3-(3-bromobenzyl)-1-tert-butyl-1H-pyrazolo[3,4-d]pyrimidin-4-amine | C16 H18 Br N5 | 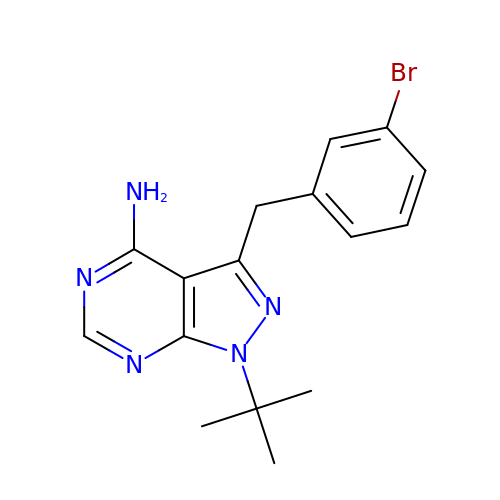FTICVONBLRGQJW-UHFFFAOYSA-N> SMKQYEHVTRDLNPEDFWEIIGELGDGAFGKVYKAQNKETSVLAAAKVIDTKSEEELEDYMVEIDILASCDHPNIVKLLDAFYYENNLWILIEFCAGGAVDAVMLELERPLTESQIQVVCKQTLDALNYLHDNKIIHRDLKAGNILFTLDGDIKLADFGVSAKNTRTIQRRDSFIGTPYWMAPEVVMCETSKDRPYDYKADVWSLGITLIEMAEIEPPHHELNPMRVLLKIAKSEPP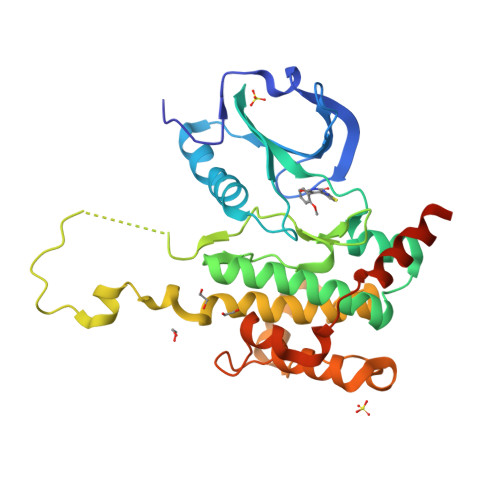TLAQPSRWSSNFKDFLKKCLEKNVDARWTTSQLLQHPFVTVDSNKPIRELIAEAKAEVTEEVEDGKE>GAMTTSESPDAYTESFGAHTIVKPAGPPRVGQPSWNPQRASSMPVNRYRPFAEEVEPIRLRNRTWPDRVIDRAPLWCAVDLRDGNQALIDPMSPARKRRMFDLLVRMGYKEIEVGFPSASQTDFDFVREIIEQGAIPDDVTIQVLTQCRPELIERTFQACSGAPRAIVHFYNSTSILQRRVVFRANRAEVQAIATDGARKCVEQAAKYPGTQWRFEYSPESYTGTELEYAKQVCDAVGEVIAPTPERPIIFNLPATVEMTTPNVYADSIEWMSRNLANRESVILSLHPHNDRGTAVAAAELGFAAGADRIEGCLFGNGERTGNVCLVTLGLNLFSRGVDPQIDFSNIDEIRRTVEYC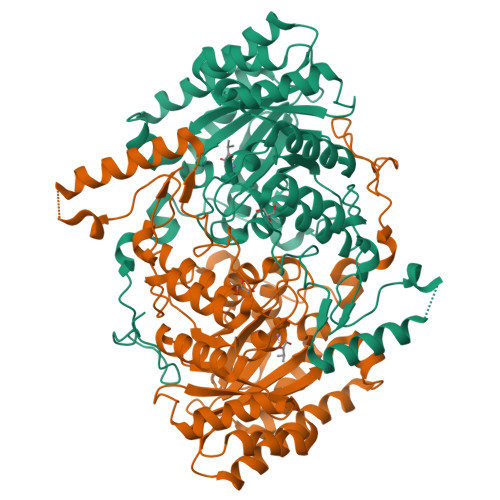NQLPVHERHPYGGDLVYTAFSGSHQDAINKGLDAMKLDADAADCDVDDMLWQVPYLPIDPRDVGRTYEAV[2x]> MDLTHFQDGRPRMVDVTEKPETFRTATAEAFVELTEEALSALEKGGVGKGDPLVVAQLAGILAAKKTADLIPLCHPLPLTGVEVRVELLKAEKRVRIEATVKTKAETGVEMEAMTACAVAALTVYDMLKAASK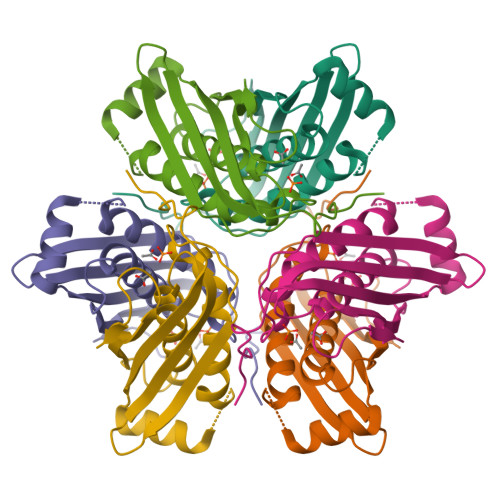GLVISQVRLLHKAGGKSGEWRREQ> SDQNVDSRDPVQLNLLYVQARDDILNGSHPVSFDKACEFAGYQCQIQFGPHNEQKHKPGFLE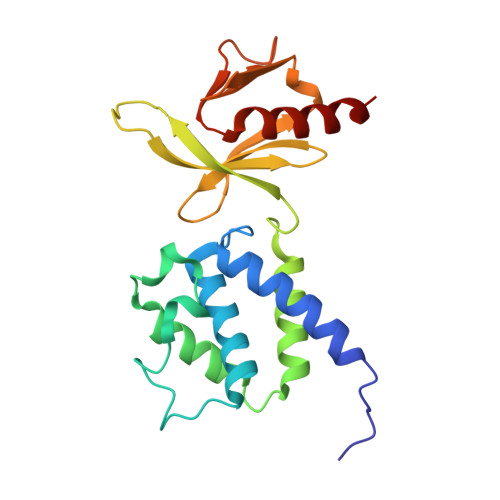LKDFLPKEYIKQKGERKIFMAHKNCGNMSEIEAKVRYVKLARSLKTYGVSFFLVKEKMKGKNKLVPRLLGITKECVMRVDEKTKEVIQEWSLTNIKRWAASPKSFTLDFGDYQDGYYSVQTTEGEQIAQLIAGYIDIIL> ETDCRWDGCSQEFDSQEQLVHH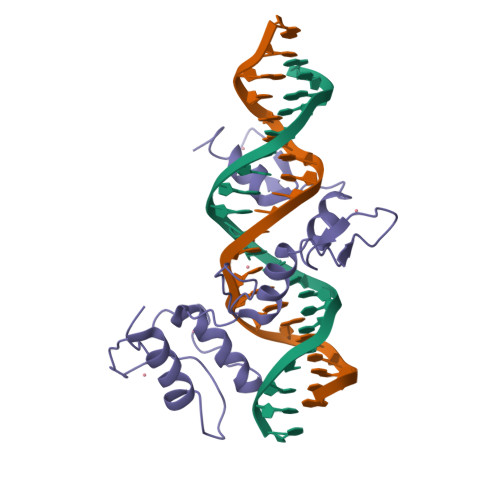INSEHIHGERKEFVCHWGGCSRELRPFKAQYMLVVHMRRHTGEKPHKCTFEGCRKSYSRLENLKTHLRSHTGEKPYMCEHEGCSKAFSNASDRAKHQNRTHSNEKPYVCKLPGCTKRYTDPSSLRKHVKTVHG>[2x]MSAPTPLAEASQIPTIPALSPLTAKQSKGNFFSSNPISSFVVDTYKQLHSHRQSLELVNPGTVENLNKEVSRDVFLSQYFFTGLRADLNKAFSMNPAFQTSHTFSIGSQALPKYAFSALFANDNLFAQGNIDNDLSVSGRLNYGWDKKNISKVNLQISDGQPTMCQLEQDYQASDFSVNVKTLNPSFSEKGEFTGVAVASFLQSVTPQLALGLETLYSRTDGSAPGDAGVSYLTRYVSKKQDWIFSGQLQANGALIASLWRKVAQNVEAGIETTLQAGMVPITDPLMGTPIGIQPTVEGSTTIGAKYEYRQSVYRGTLDSNGKVACFLERKVLPTLSVLFCGEIDHFKNDTKIGCGLQFETAGNQELLMLQQGLD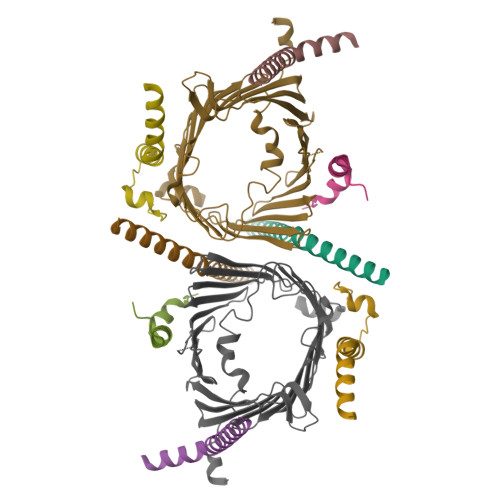ADGNPLQALPQL;>MVELTEIKDDVVQLDEPQFSRNQAIVEEKASATNNDVVDDEDDSDSDFEDEFDENETLLDRIVALKDIVPPGKRQTISNFFGFTSSFVRNAFTKSGNLAWTLTTTALLLGVPLSLSILAEQQLIEMEKTFDLQSDANNILAQGEKDAAATANRTLQVDGSPGHHHHHHHHHH[2x];>MFGLPQQEVSEEEKRAHQEQTEKTLKQAAYVAAFLWVSPMIWHLVKKQWK[2x];>[2x]MDGMFAMPGAAAGAASPQQPKSRFQAFKESPLYTIALNGAFFVAGVAFIQSPLMDMLAPQL;>[2x]MSFLPSFILSDESKERISKILTLTHNVAHYGWIPFVLYLGWAHTSNRPNFLNLLSPLPSV> VEKLKTQMLDQEELLASTRRDQDNMQAELNRLQAENDASKEEVKEVLQALEELAVNYDQKSQEVEDKTKEY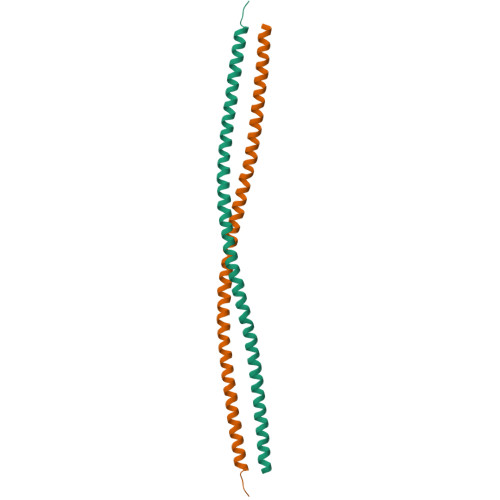ELLSDELNQKSATLASIDAELQKLKEMTNHQKKRAAEMMASLLKDLA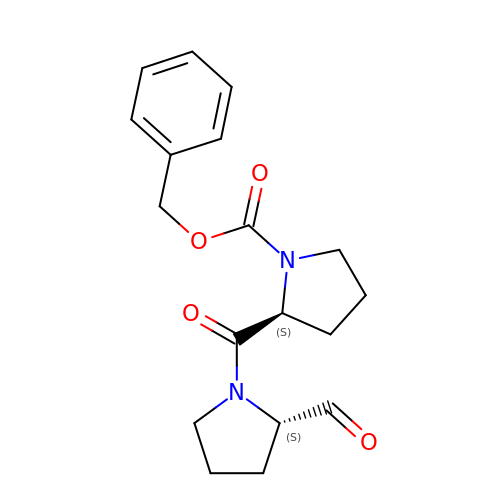N-BENZYLOXYCARBONYL-L-PROLYL-L-PROLINAL | C18 H22 N2 O4 | ORZXYSPOAVJYRU-HOTGVXAUSA-N>MNNQIFESVDHYISDLLGYEDDALLAATNSLAEAGMPAISVSPNQGKFLQLLAQLCQAKNILELGTLAGYSTIWMARALPKNGRLITLEYDPKHAAVAQKNIDRAGLTSQVQIRTGKAIDILPQLVEEGAGPFDMIFIDADKPPYTEYFQWALRLSRPGTLIVADNVIRDGKVLDENSTEPAVQGARRFNAMLGANTAVDATILQMVGVKEYDGMALAIVKLEHHHHH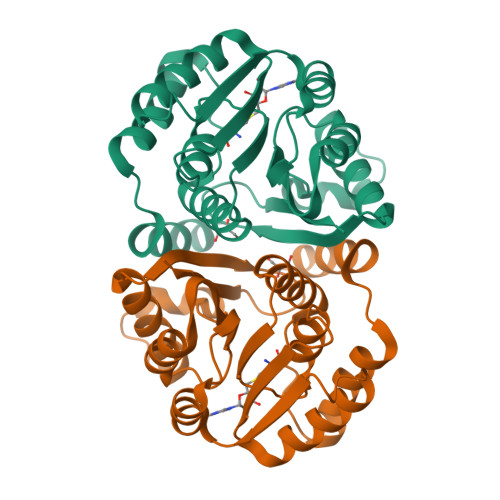H[2x]> MDTRPIGFLDSGVGGLTVVCELIRQLPHEKIVYIGDSARAPYGPRPKKQIKEYTWELVNFLLTQNVKMIVFACNTATAVAWEEVKAALDIPVLGVVLPGASAAIKSTTKGQVGVIGTPMTVASDIYRKKIQLLAPSIQVRSLACPKFVPIVESNEMCSSIAKKIVYDSLAPL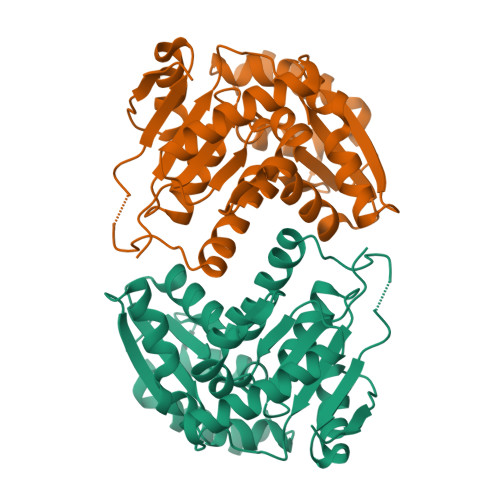VGKIDTLVLGCTHYPLLRPIIQNVMGPSVKLIDSGAECVRDISVLLNYFDINGNYHQKAVEHRFFTTANPEIFQEIASIWLKQKINVEHVTL> LPLYFGWFLTKKSSETLRKAGQVFLEELGNHKAFKKELRQFVPGDEPREKMDLVTYFGKRPPGVLHCTTKFCDYGKAPGAEEYAQQDVLKKSYSKAFTLTISA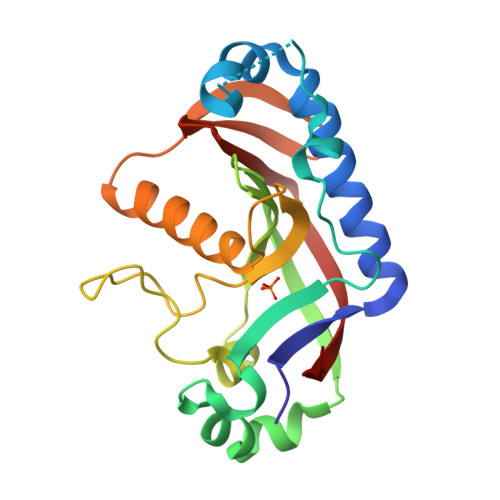LFVTPKTTGARVELSEQQLQLWPSDVDKLSPTDNLPRGSRAHITLGCAADVEAVQTGLDLLEILRQEKGGSRGEEVGELSRGKLYSLGNGRWMLTLAKNMEVRAIFTGYYG>[2x]GM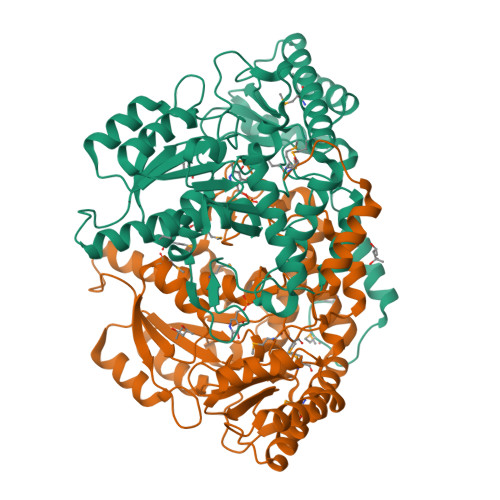RNMQEKGVSEKEILEELKKYRSLDLKYEDGNIFGSMCSNVLPITRKIVDIFLETNLGDPGLFKGTKLLEEKAVALLGSLLNNKDAYGHIVSGGTEANLMALRCIKNIWREKRRKGLSKNEHPKIIVPITAHFSFEKGREMMDLEYIYAPIKEDYTIDEKFVKDAVEDYDVDGIIGIAGTTELGTIDNIEELSKIAKENNIYIHVDAAFGGLVIPFLDDKYKKKGVNYKFDFSLGVDSITIDPHKMGHCPIPSGGILFKDIGYKRYLDVDAPYLTETRQATILGTRVGFGGACTYAVLRYLGREGQRKIVNECMENTLYLYKKLKENNFKPVIEPILNIVAIEDEDYKEVCKKLRDRGIYVSVCNCVKALRIVVMPHIKREHIDNFIEILNSIKRD N~5~-[4-(methylsulfanyl)butanimidoyl]-L-ornithine | C10 H21 N3 O2 S | 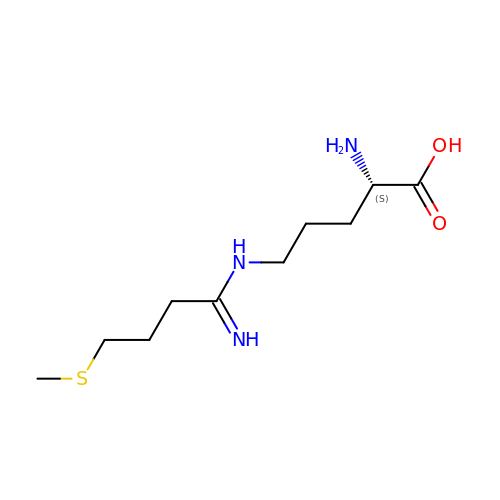BHXCYHGJTSQWOB-QMMMGPOBSA-N> SSQLHVAIVSSPGMGHLIPVLVLGNRLATHHNIKITILAITTTSSSAETEFLKKTTLTNEEKTIEIIPVPSVDISHLINSSTKIFTQLRLLVREALPKIHSTIASMTHRPDALIVDIFCTQILPIAEEFNISKYTYHPTTAWTLALAIYCQVFDKEIEGEYVELKEPLKIPGCKALRPDDVVDPLLDRSDQQYEEYVKLGKEYTDFDGILINTWEDLEP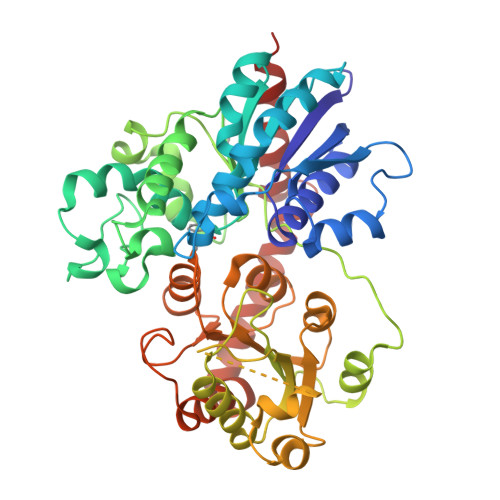ETINALRYNEKLRLLLKVPVFPIGPLRRKVETTLNDEVIQWLDKQNNESVLFVSFGSGGTLSTKQMTELAWGLELSQQKFVWVVRPPSDGDADSAYLNSAGKDTRDMSEYLPEGFLTRTKDMGLVVPMWANQVEILSHSSVGGFLTHCGWNSTVESLTNGVPMIAWPLHAEQKMNAAMLTEELGVAIRPAVLPTKKLVKREEIQGMVRILMQTKEGKRIKEKAKKLKKSAENALSDGGSSYNSICELVKDIRSREL>[3x]VEIPSSFDSRKKWPRCKS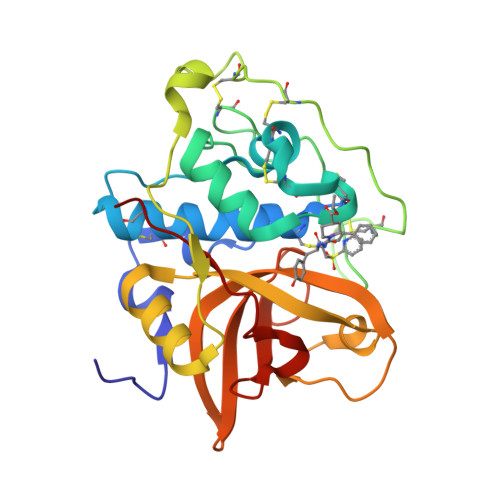IATIRDQSRCGSCWAFGAVEAMSDRSCIQSGGKQNVELSAVDLLSCCESCGLGCEGGILGPAWDYWVKEGIVTGSSKENHAGCEPYPFPKCEHHTKGKYPPCGSKIYKTPRCKQTCQKKYKTPYTQDKHRGKSSYNVKNDEKAIQKEIMKYGPVEAGFTVYEDFLNYKSGIYKHITGETLGGHAIRIIGWGVENKAPYWLIANSWNEDWGENGYFRIVRGRDECSIESEVTAGRIN(betaS)-beta-methyl-L-tryptophan | C12 H14 N2 O2 | 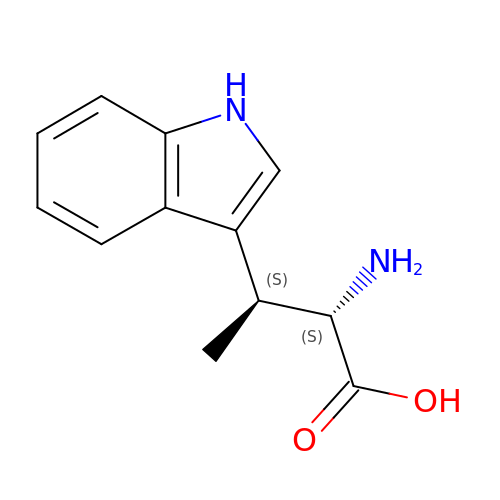CZSQAYAIWDEOSA-CPCISQLKSA-N> MGMSKPDRVVLIGVAGDSGCGKSTFLNRLADLFGTELMTVICLDDYHSLDRKGRKEAGVTALDPRANNFDLMYEQVKALKNGETIMKPIYNHETGLIDPPEKIEPNRIIVIEGLHPLYDERVRELLDFSVYLDIDDEVKIAWKIQRDMAERGHSYEDVLASIEARRPDFKAYIEPQRGHADIVIRVMPTQLIPNDTERKVLRVQLIQREGRDGFEPAYLFDEGSTIQWTPCGRKLTCSYPGIRLAYGPDTYYGHEVSVLEV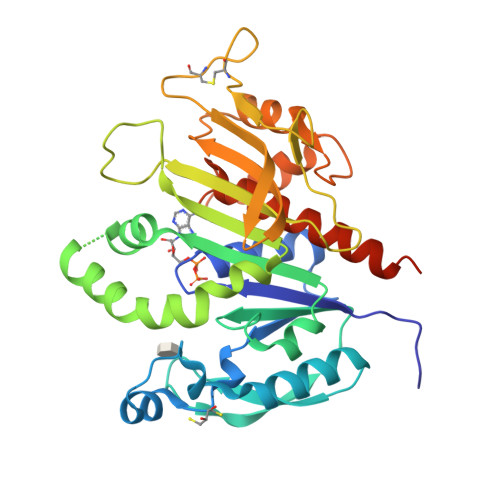DGQFENLEEMIYVEGHLSKTDTQYYGELTHLLLQHKDYPGSNNGTGLFQVLTGLKMRAAYERLTSQAAPVAASVLEHHHHHH>TGKNVNVEFDKGQNSARYS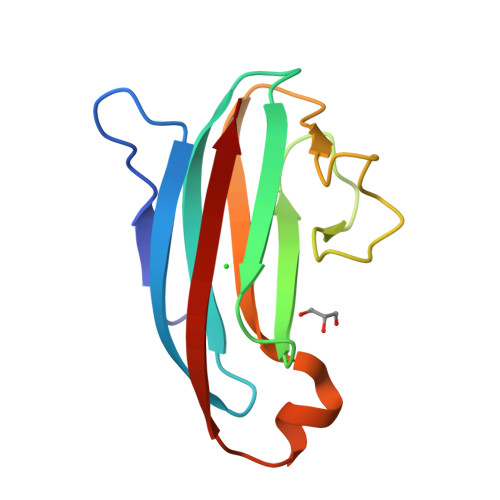GVIKGYDYDTYNFQARKGQKVHVSISNEGADTYLFGPGISDSVDLSRYSSELDGNGQYTLPASGKYELKVLQTRNEARKNKAKKYSVNIQIK[3x]>[8x]MDTKLYIDGQWVNSSSGKTVDKYSPVTGQVIGRFEAATRDDVDRAIDAAEDAFWAWNDLGSVERSKIIYRAKELIEKNRAELENIIMEENGKPVKEAKEEVDGVIDQIQYYAEWARKLNGEVVEGTSSHRKIFQYKVPYGIVVALTPWNFPAGMVARKLAPALLTGNTVVLKPSSDTPGSAEWIVRKFVEAGVPKGVLNFITGRGSEIGDYIVEHKKVNLITMTGSTATGQRIMQKASANMAKLILELGGKAPFMVWKDADMDNALKTLLWAKYWNAGQSCIAAERLYVHEDIYDTFMSRFVELSRKLALGDPKNADMGPLINKGALQATSEIVEEAKESGAKILFGGSQPSLSGPYRNGYFFLPTIIGNADQKSKIFQEEIFAPVIGARKISSVEEMYDLANDSKYGLASYLFTKDPNIIFEASERIRFGELYVNMPGPEASQGYHTGFRMTGQAGEGSKYGISEYLKLKNIY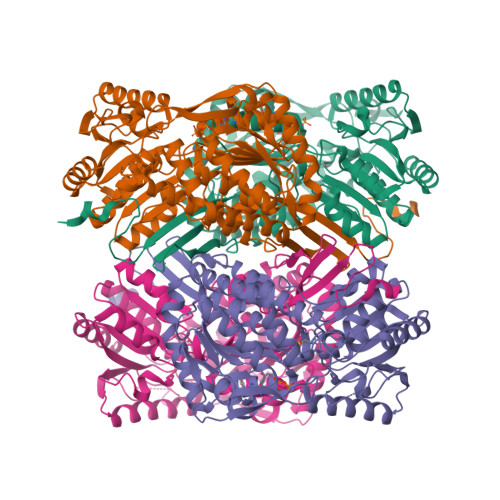VDYSGKPLHINTVRDDLFQSGRPVLGSSHHHHHH> LAPYTLPQIATKVQVKHVPGKGRCLYTKHDLEPGSIIFVETPVLVAIPSLDEELWSVLTEINDEEALELPPVWHLAAICSLTMLDDEKKKICLDKWVPDPDRAPSDDVLRVINRAGLQVHPKLYERMLMVWRYNSFGHHTEQHGLVLYNRISMMAHSCRATACWHYGEDDAFILRARVKLQAGDELTISYIGDDDLFKSTNVRREKVYGWLFTCQCVRCAAPVDNARGFRCPLCGTGAMFFKTEDGETTSSACTICQAFPTQETIQEYLDF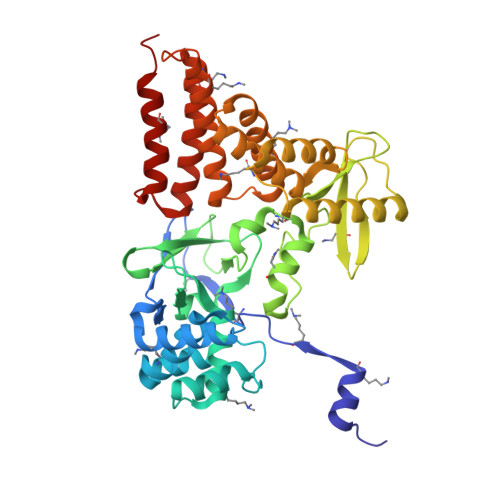EQAYVDRLAETDKSDVPDAELVYNQATRVFAQHWVLYQLHTILFEGYRDAGNSESASFHQMERIKYVSQVMPLASYTLAWLYEEMGDTMLNKAEESGPEVPAHKLNVISRHFEDAYNLLYILCGEDHDYTVAAGTKKTACEERLPAS>MPSEQRGQHRSGYGLGLSTRTQVTGYQFLARRTAMALTRWRVRMEVEPGRRQVLAVVASVSAAGVICLGALLWSFISPSGQMGESPIIADRDSGALYVRVGDTLYPALNLASARLIAGRAENPHKVRSSQIAEQPHGPMVGIPGAPSDISPTSPASSSWLVCDAVTAAQGVGAPASVTVTVIDGTPDLSGRRHVLSGSDAVVLRYGNDTWVIRQGRRSRIDAANRAVLLPLGLTPEQVKQASPMSRALYDALPVGPELAVPKVPDAGKPANFPGAPAPVGAVLVTPQISGPQQYSVVLPDGVQTISPIVAQILQNAGTPAGSMPVVVAPATLARMPVVHGLDLSAYPDSPLNVVNMKENPATCWWWEKTAGEERARTQVVSGPTVPIATSDTNKVVSLVKADNTGREADRVYYGPNYANFVVVTGNDPAASTAESLWLLSKSGVRFGVDNSREARTALGLTSTPSPAPWVALRLLAPGPMLSRADALVRHDTLPTDTNPAELAVPK[6x];>[6x]MKQGFARPTPERAPVVKPENIVLPTPLSVPPPEGKPWWLVVVGVLVVGLLVGMVGMTVASGSRLFLGAGAIFPIFMIGGVAMMMFGGRFGGQQQMSRPKLDAMRAQFMLMLDMLRETAQESADSMDANYRWFHPAPTTLAAAVGSSRMWERQPDGKDLNFGVVRVGVGMTRPEVTWGEPQNMPTDIELEPVTGKALQEFGRYQSVVYNLPKMVSLLVEPWYSLVGEREQVLGLTRAIICQLAFSHGPDHVQMIVVTSDPDRWDWVKWIPHFGDPRRRDAAGNARMVYTSVREFATEQAELFAGRGSFTPRHASSSAETPTPHHVIISDIEDPQWEYVISSEGVDGVTFFDLTGSPLWTGAPQRVLRFTDSAGVIETLPRDRDTWMVIDDNAWFFALADQMSEADAEQFAHQMAHWRLAEAYEEIGQRVVQLGARDILSYYGIDDAGEIDFNTLWSGSGRRDLLSRSRLRIPFGNRADNGELLFLDMKSLDEGGDGPHGVMSGTTGSGKSSLVRTVIASLMLAHPPEELQFVLADLKGGSAVKPFDGVPHVSRIITDLEDDQALMERFLEAMWGEIARRKEICFSAGVDGAKEYNELRARMKARGEDMPPLPMLVVVIDEFYEWFRIMPTAVDVLDSIGRQGRAYWVHLMMASQTIESRAEKLMENMGYRLVLKAQTAGAAQAAGVPNAVNLPSQAGLGYFRKSGDEIIRFQAEYLWRDYRRGSSYDGEEQAPLTHSVDYIRPQLFTTAFAPLEVSVSGPDGQSALPQVVDGEAVNGHRGGDDVDEEEEALRTPKVGTVIIDQLRQIDFEPYRLWHPPLDVPVPIDELVNRFLGRPWQQDYGTAKNLVFPIGIIDRPYKHDQPPWTVDTSGAGANVLILGAGGAGKTTALQTLICAAALTHTPEQVQFYCLAYSGTALTTVANLPHVGGVSGPTDPYGVRRTVAEVLGLVRDRKRSFLEYDVPSMEVFRRRKFGGEPGGVPDDGFGDVYLVIDNYRALAEENEVLIEQVNQIINQGPSFGVHVVATADRESELRPPVRSGFGSRVELRLAAVEDAKLVRSRFAKDVPPKPGRGMVAVNYVRLDSDPQAGLHTLVARPALGSTPDAVFESDSVAAAVRQVAAGEARPVRRLPARFGLDQLRQVAAADRRQGVGAGGIAWAISELDLQPVYLNFADNAHLMVTGRRECGRTTTLATIMSEIGRIYAPGASTAPPTSRPSAQVWLVDPRRQLLTVLGSDYVEKFAYNLDGVAAMMDDLAAALARREPPPGLSAEELLSRSWWSGPEIFLIIDDIQQLPPGFDSPLHKAAPWVTRAADVGLHVFVTRTFGGWSSAGSDPILRALHQANAPLLVMDADPDEGFIRGKMKGGPLPRGRGLLMAEDTGVFVQVAATDLRR;>[12x]MTAIVEAPQPGAEAIASPQAAVVAIMAADVQIAVVLDAHAPISVMIDPLLKVVNTRLRELGVAPLEAKGRGRWMLCLVDGTPLRPNLSLTEQEVYDGDRLWLKFLEDTEHRSEVIEHISTAVATNLSKRFAPIDPVVAVQVGATMVAVGVLLGSALLGWWRWQHESWLPAPFAAVIAVLVLTVATMILARSKTVPDRRVGDILLLSGLVPLAVAIAATAPGPVGAPHAVLGFGVFGVAAMLVMRFTGRRLGVYTALVTLCAAATAAGLARMVLLTSAVTLLTCVLLACVLMYHGAPALSRWLSGIRLPVFPSATSRWVFEARPDLPTTVVVSGGGQPTLEGPASVRDVLLRAERARSFLTGLLVGLGVLTVVCLAGLCDPHAGRRWLPLLLAAFTFGFLILRGRSYVDRWQAITLAATAVLIIAAVAVRYVLVSGSPAVLSAGVAVLVLLPAAGLTAAAVVPNTIYSPLFRKIVEWIEYLCLMPIFPLALWLMNVYEAIRYR;>MRAQRRFGLDLSWPRLTGVFLIDVAVLALVSHLPDAWQANHIAWWTGVGVAVLVTIVAVVTYRRTPLACALVARVLDRFVDPEMTLTEGCTPALDHQRRFGHDVVGIREYQGQLVAVVTVEGHEEAPSGRHRNRDAAPAWLPVEAVAARLRQFDVRLDAIDIVSVGTRRTSGRDDVSDVGVDDTGPVDARQPLDEHHTWLVLRMDPQRNVAAVAARDSVAATLAAATERLAHDLNGRRWTARPLTSSEIDDMDATVLAGLQPAHVRPRRRRLKYKQPEGYKEFVTSFWVSPRDITSETLERLWLPDTEATAVTVRLRPRHGGVEVSAWVRYHSSRRLRRSVWGGLNRLTGRQLDAVCASMPVPTRRPRLVVPARELHDGEELAVLVGQAPAPSPSPAAAR[6x]

The ESX-5 type VII secretion system is a membrane-spanning protein complex key to the virulence of mycobacterial pathogens. Key to their pathogenicity is the secretion of a wide range of virulence proteins via type VII secretion systems (T7SSs). The ESX-5 T7SS is found almost exclusively in slow growing, pathogenic mycobacteria and plays a key role in nutrient uptake and immune modulation during an infection. The importance of ESX-5 and other ESX secretion systems (ESX-1 to ESX-4) for the virulence of mycobacterial pathogens makes these membrane-spanning machineries a key target for the development of novel therapeutics.

Here, we present the high-resolution structure of the 2.1-megadalton ESX-5 core complex. Our data revealed a highly dynamic central ESX-5 pore embedded within a rigid membrane scaffold formed by six protomeric units, with a diameter ranging from 4 to 10 Å, suggesting that we captured ESX-5 in the partially open, secretion-competent state. Moreover, our structure showed an unanticipated break in symmetry between the membrane and cytoplasmic regions, with a sixfold symmetric arrangement, and the periplasmic region, which displayed a twofold symmetry. Within the TM segment, one of the main interactions required for hexamerization occurs between the TM domains of EccB5 and EccC5. We observed that the EccC5 TMH1 of each protomer interacts with the EccB5 TMH of the neighboring protomer via hydrophobic interactions and is further stabilized by the EccC5 TMH2. This domain swapping interaction was repeated in an anticlockwise fashion when viewed from the periplasm, thus generating an interlocking mechanism of next neighbor protomers within the TM section of the overall ESX-5 complex. The TMHs of EccC5 from each of the six protomers, most notably the TMH2 of one EccC5 subunit that forms a domain swapping interaction with TMH1 of the neighboring subunit, contribute to the formation of this central pore. In contrast to most other TMHs of the complex, the density of TMH2 is less well defined, which implies that this helix is more flexible and adopts a range of orientations, as indicated by our calculated ensemble model. Our results showed that the narrowest constrictions of the central pore reduce the pore diameter to slightly below 1 nm. As this pore diameter is too narrow to secrete folded substrates with an estimated width of around 2.2 nm, we hypothesize that our model, in the absence of a bound substrate, represents a gated, secretion-competent state.> YIRLY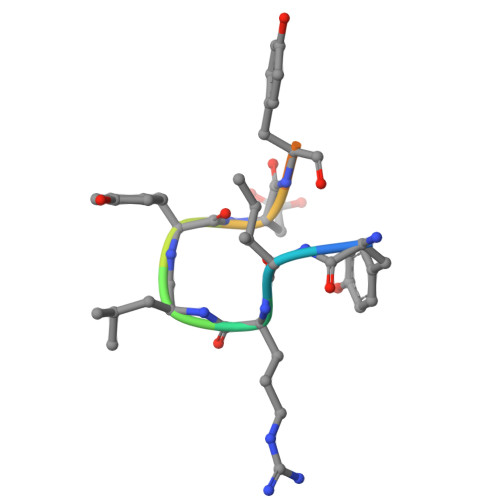DYHNC>SVDHGFLVTRHSQTTDDPQCPPGTKILYHGYSLLYVQGNERAHGQDLGTAGSCLRKFSTMPFLFCNINNVCNFASRNDYSYWLSTPEPMPMSMAPITGENIRPFISRCAVCEAPAMVMAVHSQTIQIPQCPTGWSSLWIGYSFVMHTSAGAEGSGQALASPGSCLEEFRSAPFIECHGRGTCNYYANAYSFWLATIERSEMFKKPTPSTLKAGELRTHVSRCQVCMRRT[4x];>ISIGYLLVKHSQTDQEPMCPVGMNKLWSGYSLLYFEGQEKAHNQDL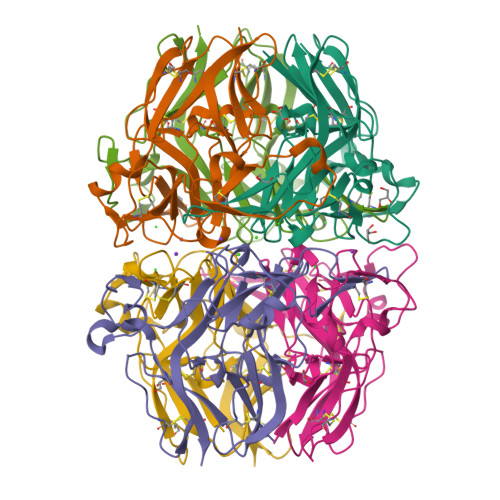GLAGSCLARFSTMPFLYCNPGDVCYYASRNDKSYWLSTTAPLPMMPVAEEDIRPYISRCSVCEAPAVAIAVHSQDVSIPHCPAGWRSLWIGYSFLMHTAAGDEGGGQSLVSPGSCLEDFRATPFIECNGARGTCHYYANKYSFWLTTIPEQSFQGTPSADTLKAGLIRTHISRCQVCMKNL[2x]Phosphotriesterase-like Lactonases (PLLs) are appealing candidates, being natural lactonases endowed with promiscuous phosphotriesterase activity. PTEs and PLLs belong to the amidohydrolase superfamily, and share the same (β/α)8 barrel topology. SsoPox exhibits high acyl-homoserine lactones and oxo-lactones hydrolysis abilities, and promiscuous, low phosphotriesterase activity. SsoPox is a very appealing candidate for the bioremediation of phosphotriesters because of its unique thermal stability, and its ability to resist aging, solvent and protease treatments.

αsB5 (V27A-I76T-Y97W-Y99F-L130P-L226V) is the only selected mutant that does not contain a substitution of position W263. In the two other mutants, αsD6 and αsB5, loop 8 could not be modeled due to the lack of electronic density, which was likely to be due to the high level of motion of this enzyme region. Analysis of the normalized thermal motion B-factor supports this hypothesis. Structures reveal that αsB5 mutations have a destabilizing effect on loop 8, as illustrated by the B factor analysis. The two selected variants, namely αsB5 and αsD6, which lost the thiono-effect have only two mutations in common: V27A and Y97W. Both residues are located relatively close to the bi-metallic active site, yet do not interact directly with the metals (V27-Fe: 6.7 Å, Y97-Co: 4.3 Å). Because W263 substitutions were previously shown to be key for increasing SsoPox’s phosphotriesterase activity, we used saturation mutagenesis to introduce W263 mutations to the background of αsB5. The best selected mutants against paraoxon were found to be αsB5-W263I/L/M. Surprisingly, none of these mutants demonstrated an increase in phosphotriesterase activity in comparison with αsB5, but rather a decrease in activity. For example, with ethyl-paraoxon as a substrate, W263M and αsB5 produce a catalytic efficiency improvement of 14 and 67-fold, respectively, while the combination αsB5-W263M increases activity only 11-fold. The destabilizing effect of these mutations can also be observed on the overall enzyme stability, with αsB5, W263M, αsB5-W263M exhibiting Tm values of 70.4 °C, 85.3 °C and 69.1 °C, respectively, as compared to 106 °C for the wt enzyme.

>MRIPLVGKDSIESKDIGFTLIHEHLRAFSEAVRQQWPHLYNEDEEFRNAVNEVKRAMQFGVKTIVDPTVMGLGRDTRFMEKVVKATGINLVAGTGIWIFIDLPFYFLNRSIDEIADLFIHDIKEGIQGTPNKAGFVKIAADEPGITKDVEKVIRAAAIANKETKVPIITHSNAHNNTGLEQQRILTEEGVDPGKILIGHLGDTDNIDYIKKIADKGSFIGLDRYGVDLFLPVDKRNETTLRLIKDGYSDKIMISHDYCCTIDWGTAKPEYKPKLAPRWSITLIFEDTIPFLKRNGVNEEVIATIFKENPKKFFS[4x]> MHHHHHHSTSVDLGTENLYFQSNAEERAAGARPSATQTTGTATEPFHGPHQAGIATPPQAHAVFLGLDLRKGTGRKELGRLMRLLTDDARRLTQGRPALADPEPDLAPLPSRLTFTFGFGPGLFKAAGLEKQRPEGLRPLPPFKVDRLEDRWSGGDLLVQICCDDPITLAHALRMTVKDARAFTRVRWVQRGFRRSPGVQSSGATQRNLMGQLDGTVNPVPGTADFDQAVWVQDGPEWLRGGTTLVLRRIRMELEKWDEADPAGKEFAVGRRLTSGAPLTGRHEHDEPDFDAVDSAGFPVIAENAHIRLAHVDSPRLRMLRRPYNYDEGLTADGRSDAGLLFAAYQADIDRQFIPVQRRLDEGGDLLNLWTTPIGSAVFAIPPGCDENGWIGQGLL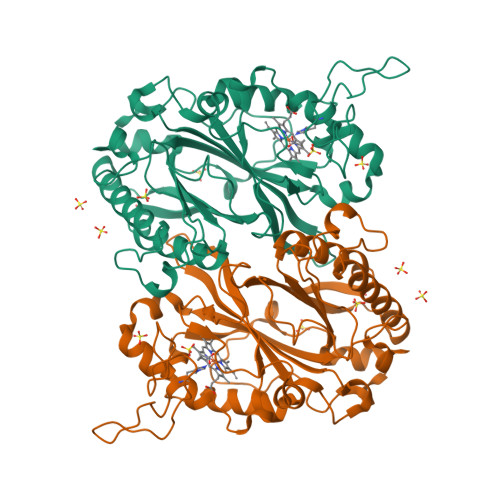G>HHHHHHFNLPP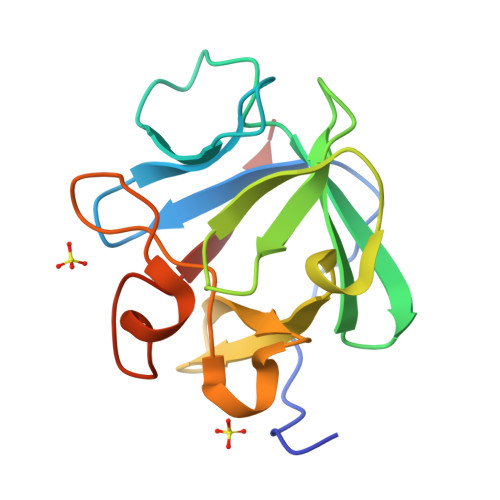GNYKKPKLLYCSNGGHFLRILPDGTVDGTRDRSDQHIQLQLSAESVGEVYIKSTETGQYLAMDTDGLLYGSQTPNEECLFLERLEENHYNTYISKKHAEKNWFVGLKKNGSIKRGPRTHYGQKAILFLPLPVSSD[2x]>AAFKPEELRQALMPTLEALYRQDPESLPFRQPVDPQLLGIPDYFDIVKNPMDLSTIKRKLDTGQYQEPWQYVDDVWLMFN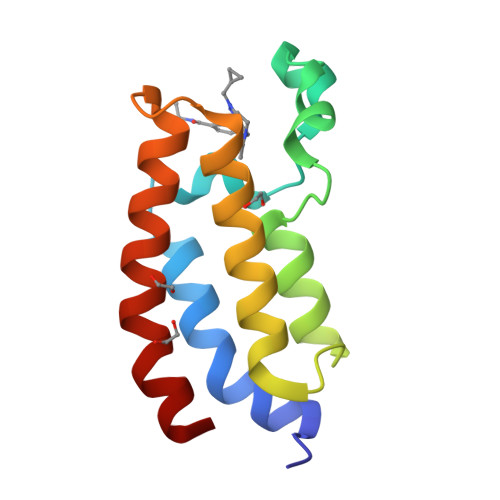NAWLYNRKTSRVYKFCSKLAEVFEQEIDPVMQAL[3x]> DPYWAYSGAYGPEHWVTSSVSCGGSHQSPIDILDHHARVGDEYQELQLDGFDNESSNKTWMKNTGKTVAILLKDDYFVSGAGLPGRFKAEKVEFHWGHSNGSAGSEHSVNGRRFPVEMQIFFYNPDDFDSFQTAISENRIIGAMAIFFQVSPRDNSALDPIIHGLKGVVHHEKETFLDPFILRDLLPASLGS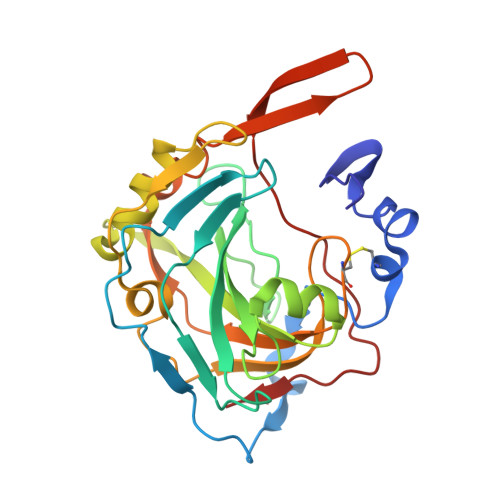YYRYTGSLTTPPCSEIVEWIVFRRPVPISYHQLEAFYSIFTTEQQDHVKSVEYLRNNFRPQQALNDRVVSKS4-[6-(1H-imidazol-1-ylmethyl)-7-methoxy-2,4-dihydroindeno[1,2-c]pyrazol-3-yl]benzonitrile 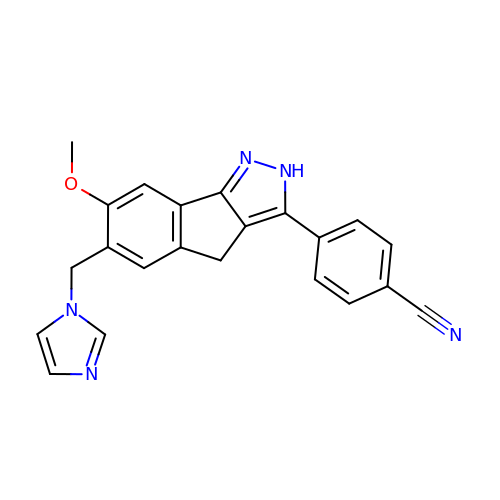| C22 H17 N5 O | XEPCYHKWASJTHM-UHFFFAOYSA-N>[4x]MAHHHHHHVDDDDKMQDRMYQRFLRQHVDPDATGGNDAYCNLMMQRRKMTSHYCKRFNTFIHEDIWN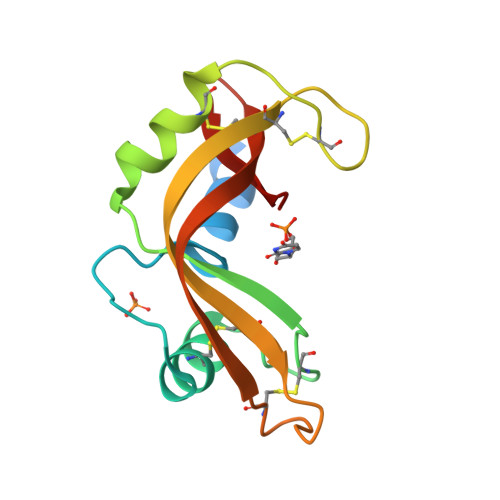IRSICSTSNIQCKNGQMNCHEGVVKVTDCRETGSSRAPNCRYRAMASTRRVVIACEGNPEVPVHFDK>MHDQRVHAERDPLDPQAHGLTITRIETIPMVAPLAREFRGSHYHMTHRATIVTRVHTDAGIIGEAYTGDEHETMFDIDRIIHEELAPTLIGQDAMAIERLWDSGYKVTFDILRDRRLGLVALAAVNTAIWDAVGKALKMPLWKLWGGYRNELPMIAIGGYYGEPLGSIADEMHNYQELGLAGVKFKVGGLSAAEDAARITAAREAAGDDFIICIDANQGYKPAVAVDLSRRIADLNIRWFEEPVEWHNDKRSMRDVRYQGSVPVCAGQTEFSASGCRDLMETGAIDVCNFDSSWSGGPTAWLRTAAIATSYDVQMGHHEEPQVSTHLLASQPHGTIAECFHPDRDPFWWNMITNRPKLNNGTLTLSDRPGLGWDLNWDYIDQ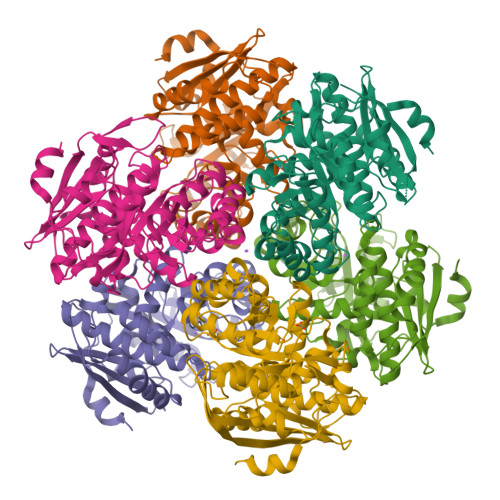YRVSKD[6x]>GMPIDTPTDASPADGSASDTVFFGIMSGLELGTFVPGQRLVETDLVAHFGVGRNSVREALQRLAAEGIVDLQRHRGAVIRRLSLQETLDVLDVAERMTGLLARAATRGSGNQPQVQALRASVQALVAAEKAQDGETFSNARRHFYRTLLEMGDNRELRRLFPTIHMPIVHAQHRLASLRQMRLDDYRRIATAVLAGEPDAA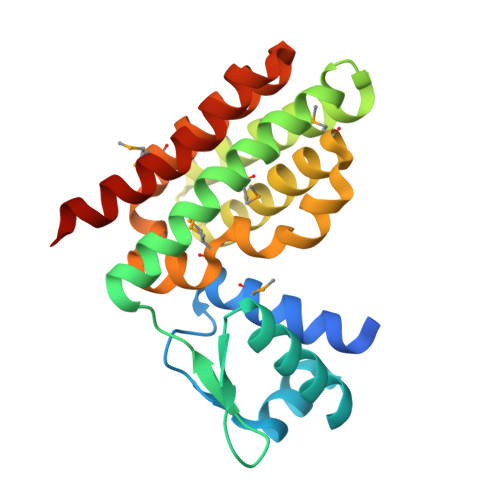EAAGAAHVKNVRGAILDRQPA[2x]> VTKPTIAAVGGYAMNNGTGTTLYTKAADTRRSTGSTTKIMTAKVVLAQSNLNLDAKVTIQKAYSDYVVANNASQAHLIVGDKVTVRQLLYGLMLPSGCDAAYALADKYGSGSTRAARVKSFIGKMNTAATNLGLHNTHFD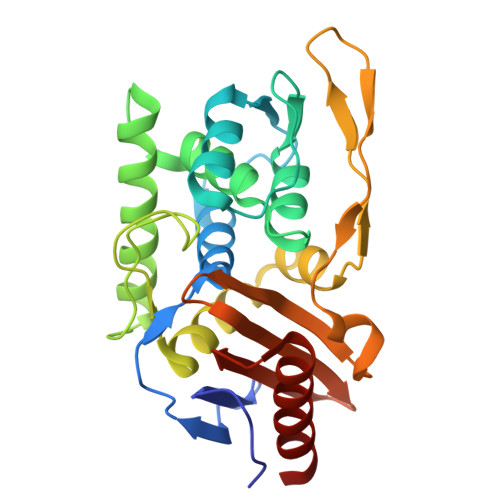SFDGIGNGANYSTPRDLTKIASSAMKNSTFRTVVKTKAYTAKTVTKTGSIRTMDTWKNTNGLLSSYSGAIGVKTGSGPEAKYCLVFAATRGGKTVIGTVLASTSIPALESDATKIMNYGFAL>SKELLAEYQDLTFLTKQEILLAHRRFCELLPQEQRSVESSLRAQVPFEQILSLPELKANPFKERICRVFSTSPAKDSLSFEDFLDLLSVFSDTATPDIKSHYAFRIFDFDDDGTLNREDLSRLVNCLTGEGEDTRLSASEMKQLIDNILEESDIDRDGTINLSEFQHVISRSPD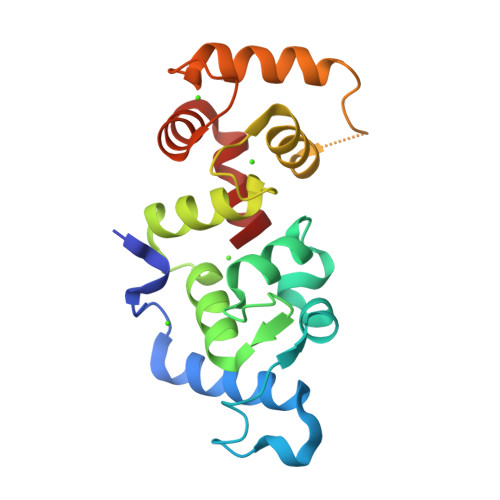FASSFKIVL[2x]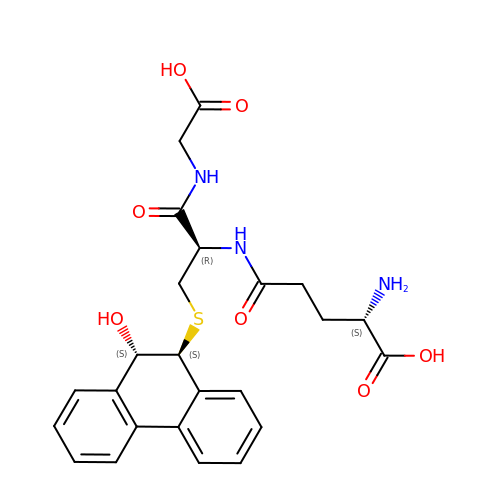L-gamma-glutamyl-S-[(9S,10S)-10-hydroxy-9,10-dihydrophenanthren-9-yl]-L-cysteinylglycine | C24 H27 N3 O7 S | JNNIZILNBMPOAC-GPHNJDIKSA-N ethyl 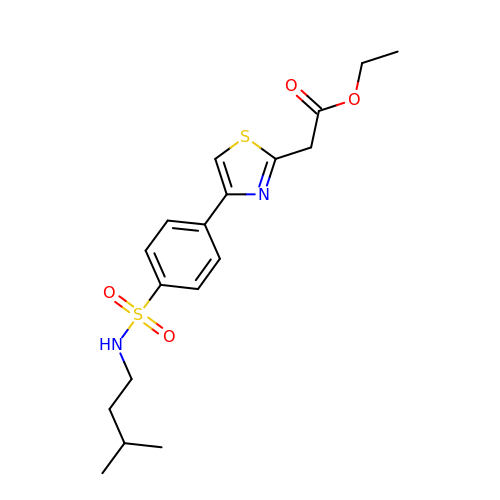2-[4-[4-(3-methylbutylsulfamoyl)phenyl]-1,3-thiazol-2-yl]ethanoate | C18 H24 N2 O4 S2 | BNWOHTVYARXZJA-UHFFFAOYSA-N> M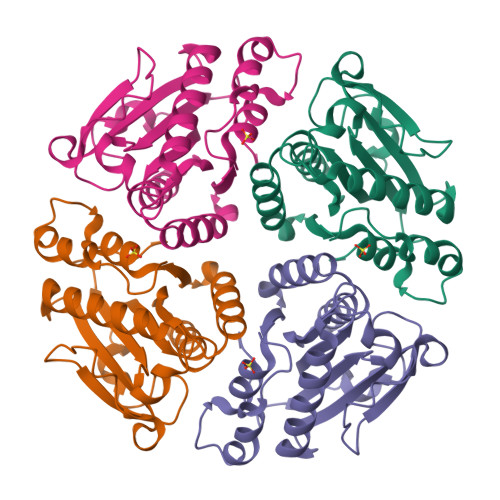AHHHHHHMSRLLKHYGSCKTAFFCCDIQEKFMGRIANSANCVFVANRFAGLHTALGTAHSVYIVTEQYPKGLGATSADIRLPPDAHVFSKKRFAMLVPQVMPLVDLPEVEQVVLWGFETHVCILQTAAALLDMKKKVVIAVDGCGSQSQGDHCTAIQLMQSWSGDGCYISTSESILMQLLKDASDPVFKTIAPLMKQTHPIRI AChBP is a soluble, highly conserved homolog of the nAChR extracellular domain (ECD) in mollusks such as the Californian sea hare (Aplysia californica) and can therefore be used as a surrogate for crystallography and binding studies. Cytisine, which is structurally related to nicotine, is a potent agonist at neuronal nAChRs but differs in displaying only partial agonist activity at α4β2 nAChRs, the high-affinity nicotine subtype. In this study, we sought to compare the binding parameters and structural interactions of cytisine and ligand 4 using acetylcholine-binding protein (AChBP).

The monoclinic crystal has two pentameric assemblies in the asymmetric unit. A high degree of noncrystallographic symmetry is evident even though NCS restraints were released in the refinement calculations. Electron density for the ligand is well defined in all ten binding sites and they refined with average B factors less than or close to the values noted for their associated subunits. The Tyr110 OH group and the carbonyl backbone of Trp164 accept hydrogen bonds from the secondary amine of the ligand, indicating the presence of a protonated group. The alignment and distances of between 4.6 and 4.2 Å of the aromatic groups on Trp164 and Tyr212, respectively, from the nitrogen suggest that cation–π interactions contribute to binding. The ligand carbonyl group accepts a hydrogen bond, with a distance of 2.7 Å, donated from a water molecule that then bridges to Ile135 (via the carbonyl) and Ile123 (via the amide) on the complementary side of the binding site. The 3-hydroxylpropyl substituent interacts with Val125, Ile135, the Cys207–Cys208 disulfide, the side chain of Met133 and the main chain of Phe134. The hydroxyl residue on 4 is directed out of the binding site, forming hydrogen bonds to two well ordered water molecules, which in turn interact with other waters and glycerol. In the AcAChBP–4 complex we note that the 3-hydroxylpropyl substituent appears to force the Met133 side chain to adopt different rotamers and thus avoid steric clash. There is only a minor perturbation of the protein structure at the side chain of Met133, where a steric clash is likely to contribute to the reduced affinity of 4 compared with the parent compound.

>MLVSVYLALLVACVGQAHSQANLMRLKSDLFNRSPMYPGPTKDDPLTVTLGFTLQDIVKVDSSTNEVDLVYYEQQRWKLNSLMWDPNEYGNITDFRTSAADIWTPDITAYSSTRPVQVLSPQIAVVTHDGSVMFIPAQRLSFMCDPTGVDSEEGVTCAVKFGSWVYSGFEIDLKTDTDQVDLSSYYASSKYEILSATQTRQVQHYSCCPEPYIDVNLVVKFRERRAGNGFFRNLFDENLYFQGHHHHHH[10x]>[3x]MKRREVLQTAASALVGALSVSTFSSYAAKNTGLALKSVDATAIPKGDVPILTPENVYAMPPQFWQNFQGKLWIGRAGSDARQPGNQIPVFLRDANGNLAQITQPITLNKGNFDQFVKDNAALIANPSHAMALEDSNGQTVFNIPDVSQPGQAAFSQRLAQPAGYQLIGEIPSVDDLRKTRPLFEGAKIKLKSWHPGLEVGGGEFVGSFQPAQDDQGVIFSGDGFHWRRVVDDYNRLSLFDFGAIADGKTDSAPAIKAMYQWSQQSDQPICVQFPAGTFFVTGCDFGEEQRRFFRISGAMVNFGYFPATTIVSDGQSPFVFEVSARWVEISNLIFNGNTDTKPNRQGLLRNTCPGGQFFRGACLRFNNVGGTALSLLDTLDCKIDQWYASACTGDVIQAGWSGQKKGNWDHSTAIELSNFNAQHCKGGKVLNLPRCSQSLIHNGWIEHCDNPGDISNGQWIIDALSLEDCKNPLIAWHSRLNTRQTNLQSGSWIDNSEQGDRWLSAWEMGSTRVESYGVAIDGSLKYNYLTSRWLLENNTSQPVWYELANLYSPTVGDSWEIEVFGQSQFNNGTDSEPLMNLIDGRNTGGRAVIHVQRKKDHAEASWSAEGSSPVLDVRYVAKTDTDTQVFIRLAGWTPSAAIMIKSTAKDRFVTGRCARVDAKMAKATPDSGSHAAPQRFSLHNGKAGVGANEQGDLLLASRALSADNVDTRKPEGFVSVVINGKTVALPYFAIKA

The plant pathogen Pantoea stewartii (P. stewartii) encodes the protein WceF within its EPS synthesis cluster. In this work, we show that WceF is a glycosidase active on stewartan, the main P. stewartii EPS biofilm component. WceF has remarkable structural similarity with bacteriophage tailspike proteins (TSPs). WceF is a stewartan hydrolase and produces oligosaccharides, corresponding to single stewartan repeat units.

We recombinantly expressed, purified, and crystallized WceF lacking the N-terminal 28 amino acids of the Tat-signal peptide that encodes for export via the Tat-pathway for folded proteins. We solved its crystal structure to 2.55 Å resolution, using a selenomethionine variant for phasing. WceF residues 34 to 736 were resolved in the electron density. As confirmed by size-exclusion chromatography, WceF is a native homotrimer of about 200 kDa. Each peptide chain is composed of an N-terminal head domain, a neck domain, the central right-handed parallel β-helix domain followed by a short triple β-helix, a β-sandwich, and a C-terminal stem domain. The head domain (residues 34–146) is made of two β-sheets containing four antiparallel β-strands flanked by three α-helices. A five-stranded Greek-key motif surrounding one α-helix then forms the neck domain (residues 166–229) of WceF. The central body of WceF is formed by a large three-stranded β-helix (residues 236–514) of eight complete rungs capped by an N-terminal α-helix (residues 252–265). At the C-terminus of the β-helix, the chain makes a β-hairpin turn and two 120° kinks that form two turns of a triple β-helix in the native trimer (residues 517–531). The intertwined chains then again separate and individually form a β-sandwich domain with a jelly roll fold composed of eight antiparallel β-strands arranged in two four-stranded sheets (residues 531–667).> G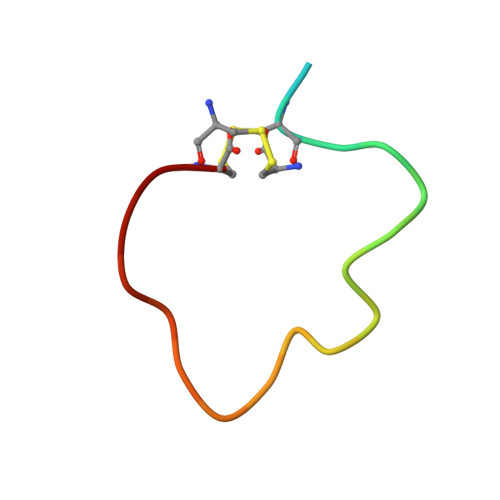LSKGCFGLKLDRIGSMSGLGC>MDGSGEQPRGGGP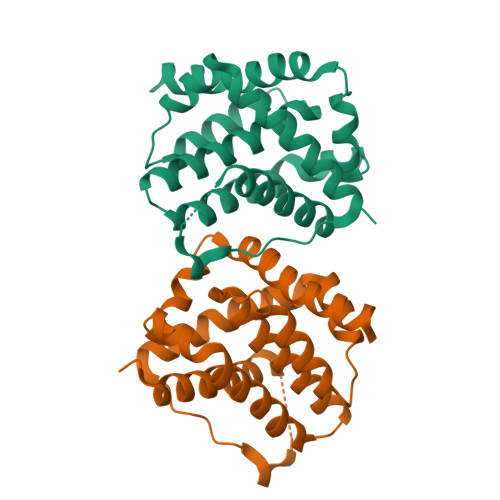TSSEQIMKTGALLLQGFIQDRAGRMGGEAPELALDPVPQDASTKKLSECLKRIGDELDSNMELQRMIAAVDTDSPREVFFRVAADMFSDGNFNWGRVVALFYFASKLVLKALCTKVPELIRTIMGWTLDFLRERLLGWIQDQGGWDGLLSYFGTGTWQTVTIFVAGVLTASLTIWKKMG[2x]> NEVSVIKEGWLHKRGEYIKTWRPRYFLLKSDGSFIGYKERPEAPDQTLPPLNNFSVAECQLMKTERPRPNTFVIRCLQWTTVIERTFHVDSPDEREEWMRAIQMVANSLKQRAAAEDPMDYKCGSPSDSSTTEEMEVAVSKARAKVTMNDFDYLKLLGKGTFGKVILVREKATGRYYAMKILRKEVIIAKDEVAHTVTESRVLQNTRHPFLTALKYAFQTHDRLCFVMEYANGGELFFHLSRERVFTEERARFYGAEIVSALEYLHSRDVVYRDIKLENLMLDKDGHIKITDFGLCKEGISDGATMKTFCGTPEYLAPEVLEDNDYGRAVDWWGLGVVMYEMMCGRLPFYNQDHERLFELILMEEIRFPRTLSPEAKSLLAGLLKKDPKQRLGGGPSDAKEVMEHRFFLSINWQDVVQKKLLPPFKPQVTSEVDTR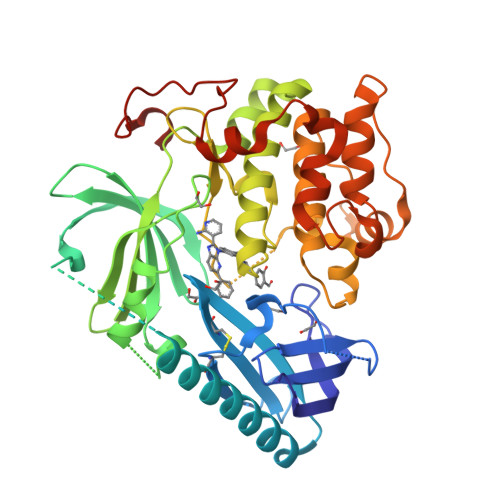YFDDEFTAQS> MTNIIQADEPTTLTTNALDLNSVLGKDYGALKDIVINANPASPPLSLLVLHRLLCEHFRVLSTVHTHSSVKSVPENLLKCFGEQNKKQPRQDYQLGFTLIWKNVPKTQMKFSIQTMCPIEGEGNIARFLFSLFGQKHNAVNATLIDSWVDIAIFQLKEGSSKEKAAVFRSMNSALGKSPWLAGNELTVADVVLWSVLQQIGGCSVTVPANVQRWMRSCENLAPFNTALKLLKLEHHHH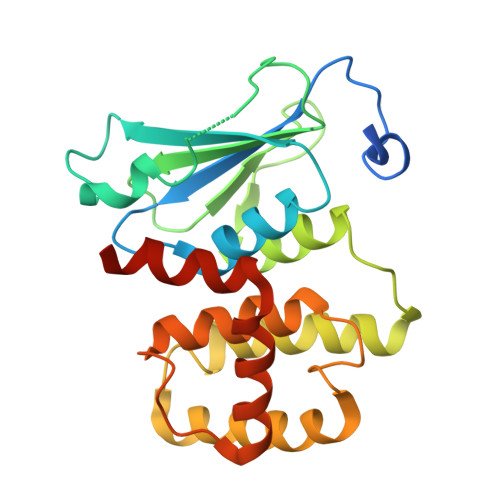HH>MSINLHSAPEYDPSYKLIQLTPELLDIIQDPVQNHQLRFKSLDKDKSEVVLCSHDKTWVLKQRKHSNTVLLMREFVPEQPITFDETLLFGLSKPYMDVVGFAKTESEFETRETHGELNLNSVPIYNGELDFSDKIMKRSSTKVIGTLEELLENSPCSALEGISKWHKIGGSVKDGVLCILSQDFLFKALHVLLMSAMAESLDLQHLNVEDTHHAVGKDIEDEFNPYTREIIETVL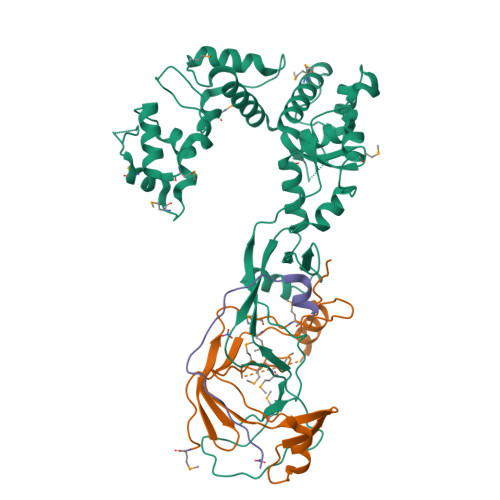NKFAVQEQEAENNTWRLRIPFIAQWYGIQALRKYVSGISMPIDEFLIKWKSLFPPFFPCDIDIDMLRGYHFKPTDKTVQYIAKSTLPMDPKERFKVLFRLQSQWDLEDIKPLIEELNSRGMKIDSFIMKYARRKRLGKKTVVTSR[2x];>[2x]MPSVDIDASQWQKLTQSREKQTTVITPLGMMMLEIQGELELPKDFASLARRDSPNEGRFSEQDGETLIRFGSLQIDGERATLFVGKKQRLLGKVTKLDVPMGIMHFNSKDNKVELVDVMKYKVIFKDRPLPIM;>[2x]TVKIWVKYNEGFSNAVRKNVTWNNLWE> MHHHHHHHHPDLGTGSENLYFQGAMADQVQDMYYLSPMQEGMLFHAILNPGQSFYLEQITMKVKGSLNIKCLEESMNVIMDRYDVFRTVFIHEKVKRPVQVVLKKRQFQIEEIDLTHLTGSEQTAKINEYKEQDKIRGFDLTRDIPMRAAIFKKAEESFEWVTSVHHIILDGWCIGIVVQDLFKVYNALREQKPYSLPPVKPYKDYIKWLEKQDKQASLRYWREYLEDFEGQTTFAEQRKKQKDGYEPKELLFSLPEAETKAFTELAKSQHTTLSTALQAVWSVLISRYQQSGDLAFGTVVSGRPAEIKGVEHMVGLFINVVPRRVKLSEGITFNDLLKQLQEQSLQSEPHQYVPLYDIQSQADQPKLIDHIIVFENYPLQDAKNEESSENGFDMVDVHVFEKSNYDLNLMASPGDEM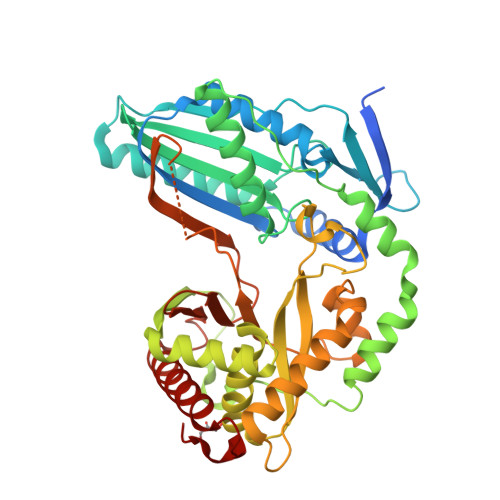LIKLAYNENVFDEAFILRLKSQLLTAIQQLIQNPDQPVSTINI>MIKIKLTHPDCMPKIGSEDAAGMDLRAFFNDLRAIAPGKSLMIDTGVAVEIPRGWFGLVVPRSSLGKRHLMIANTAGVIDSDYRGTIKMNLYNYGSEMQTLENFERLCQLVVLPHYSTHNFKIVDELEETIRGEGGFGSSGSK[3x]

Deoxyuridine triphosphate nucleotidohydrolases (dUTPases, or Duts) are produced by most living organisms as part of their pyrimidine biosynthesis networks. Their role is to eliminate excess dUTP, which can be mistakenly incorporated into DNA by DNA polymerases, since most of them cannot distinguish between dUTP and dTTP. In addition, dUTPases provide the dTTP precursor, dUMP. In this study, we demonstrate for the first time that the homotrimeric dUTPase of bacteriophage T5 performs an additional, non-enzymatic function in the virus’s life cycle.

To test our hypothesis, the next mutant T5 phage T5dut(Δloop), with a dUTPase sequence 28-FFGTNPAADL-37 reduced to 28-FFNDL-32, was obtained. To confirm that the loop reduction retains overall folding, without global changes, we obtained the mutant form T5DutΔloop structure (2.1 Å). A comparison of the crystal structures of wild-type T5Dut and its mutant form revealed no significant changes in the overall folding of the protein, except for in the mutated region. The superimposition of the wild-type and mutant forms, with an RMSD of 0.31 Å for the Cα atoms, shows the nearly identical folding of these proteins, with the only difference being observed in the region of interest. Moreover, this change in the amino acid sequence of T5 phage Dut had no impact on its enzymatic activity, specifically the hydrolysis of dUTP, as shown in the curve. The mutant phage T5dut(Δloop) did not differ from the previously obtained mutant T5dut-am in terms of its main growth characteristics. Reducing the size of this loop has dramatic consequences for the development of the phage T5i n E. coli cells, which are similar to those obtained with the complete removal of Dut. The results of these experiments clearly demonstrate that the short segment of the polypeptide chain, consisting of six amino acid residues (30-GTNPAA-35), is responsible for carrying out an additional function of T5Dut.> MVAKGRIIRVTGPLVVADGMKGAKMYEVVRVGELGLIGEIIRLEGDKAVIQVYEETAGVRPGEPVVGTGASLSVELGPGLLTSIYDGIQRPLEVIREKTGDFIARGVTAPALPRDKKWHFIPKAKVGDKVVGGDIIGEVPETSIIVHKIMVPPGIEGEIVEIAEEGDYTIEEVIAKVKTPSGEIKELKMYQRWPVRVKRPYKEKLPPEVPLITGQRVIDTFFPQAKGGTAAIPGAFGSGKTVTQHQLAKWSDAQVVIYIGCGERGNEMTDVLEEFPKLKDPKTGKPLMERTVLIANTSNMPVAAREASIYTGITIAEYFRDMGYDVALMADSTSRWAEALREISGRLEEMPGEEGYPAYLASKLAEFYERAGRVVTLGSDYRVGSVSVIGAVSPPGGDFSEPVVQNTLRVVKVFWALDADLARRRHFPAINWLTSYSLYVDAVKDWWHKNIDPEWKAMRDKAMALLQKESELQEIVRIVGPDALPERERAILLVARMLREDYLQQDAFDEVDTYCPPEKQVTMMRVLLNFYDKTMEAINRGVPLEEIAKLPVREEIGRMKFERDVSKIRSL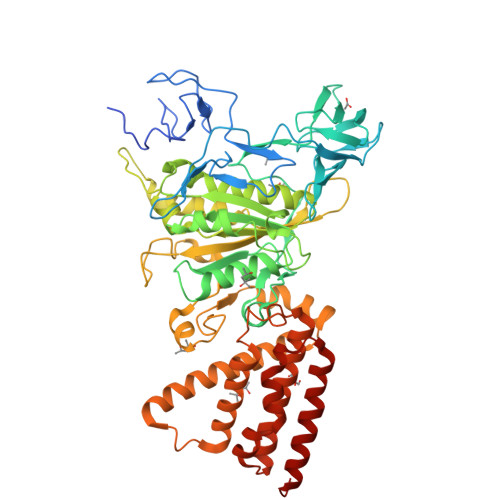IDKTNEQFEELFKKYGA> IVGGTASVRGEWPWQVTLHTTSPTQRHLCGGSIIGNQWILTAAHCFYGVESPKILRVYSGILNQSEIKEDTSFFGVQEIIIHDQ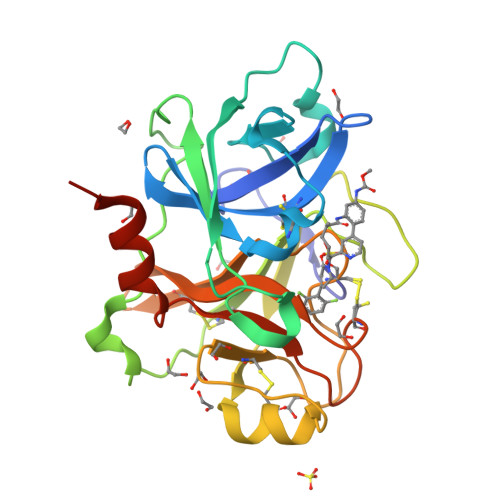YKMAESGYDIALLKLETTVGYGDSQRPICLPSKGDRNVIYTDCWVTGWGYRKLRDKIQNTLQKAKIPLVTNEECQKRYRGHKITHKMICAGYREGGKDACKGDSGGPLSCKHNEVWHLVGITSWGEGCAQRERPGVYTNVVEYVDWILEKTQAVHHHHHH> ASVSAGNSRLLGFDSIPAATTDTISLPKGYKSSVLISWGQPLHKNGPAFDPSGNGTAAAQEVQFGDNNDGMSLFEFPGEKNRALMAINNEYTNYRYLYPHGGMPQSAEDVRKALACEGVSVIEVQRKNGQWQFVQGSRYNRRIHGNSPLRISGPAAGHELMKTSADKHGKKVLGTFQNCANGKTPWGTYLTCEENFTDCFGSSNAQQQFDPAQKRYGVSAASREINWHPFDPRFDMAKN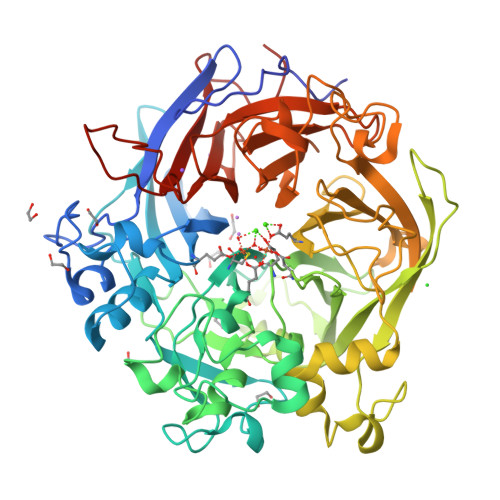PNELNRHGWVVEIDPFDPQSTPVKRTALGRFKHENAALAETDDGRAVVYMGDDERGEFIYKFVSRDKINHRNAKANRDILDHGTLYVARFDAGDGNPDHPKGQGQWIELTHGKNGIDASSGFADQAEVLIHARLAASVVGATRMDRPEWIVVSPKDGQVYCTLTNNAKRGEDGQPVGGPNPREKNVYGQILRWRTDRDDHASKTFAWDLFVVAGNPSVHAGTPKGGSSNITPQNMFNSPDGLGFDKAGRLWILTDGDSSNAGDFAGMGNNQMLCADPATGEIRRFMVGPIGCEVTGISFSPDQKTLFVGIQHPGENGGSTFPEHLPNGKPRSSVMAITREDGGIVGAHHHHHH3-[4-(aminomethyl)phenyl]-2-methyl-6-[[4-oxidanyl-1-[(3~{R})-4,4,4-tris(fluoranyl)-3-phenyl-butanoyl]piperidin-4-yl]methyl]pyrazolo[4,3-d]pyrimidin-7-one | C29 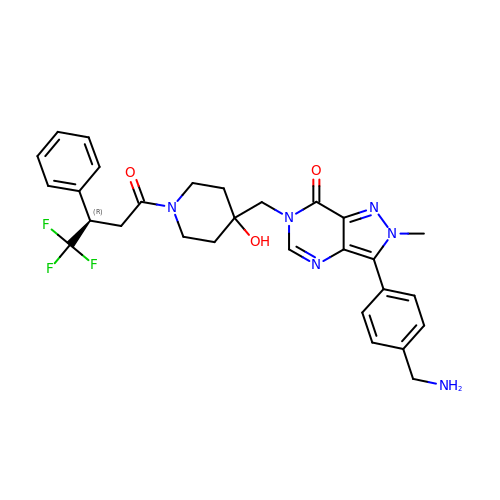H31 F3 N6 O3 | RLPQYKGBXQQARM-JOCHJYFZSA-N4-[(4-aminophenyl)amino]pyrido[2,3-d]pyrimidin-5(6H)-one | C13 H11 N5 O | 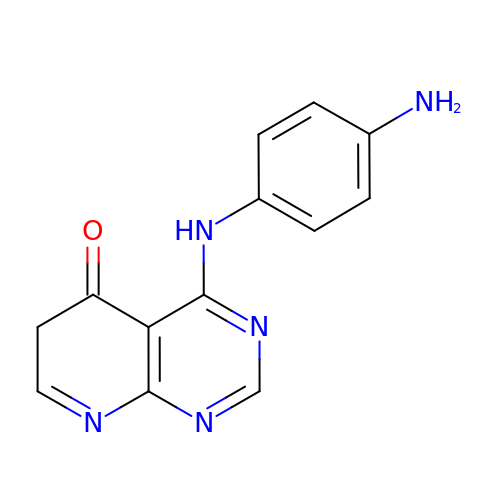FWUUBTREFIXWHX-UHFFFAOYSA-N> MLRDLFDRAVVLSHYIHNLSSEMFSEFDKRYTHGRGFITKAINSCHTSSLATPEDKEQAQQMNQKDFLSL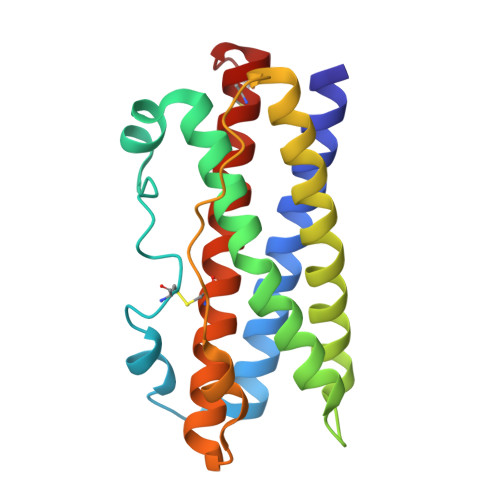IVSILRSWNEPLYHLVTEVRGMQEAPEAILSKAVEIEEQTKRLLERMELIVSQVHPETKENEIYPVWSGLPSLQMADEESRLSAYYNLLHCLRRDSAKIDNYLKLLKCRIIHNNNC decanoyl-CoA | C31 H54 N7 O17 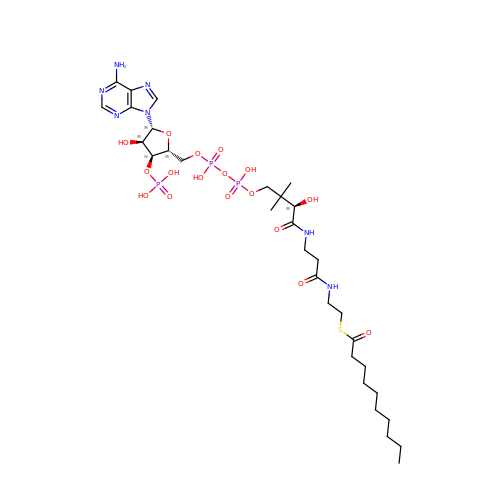P3 S | CNKJPHSEFDPYDB-HSJNEKGZSA-N> MASPPPFHSQKLPGEYFRYKGVPFPVGLYSLESISLAENTQDVRDDDIFIITYPKSGTTWMIEIICLILKEGDPSWIRSVPIWERAPWCETIVGAFSLPDQYSPRLMSSHLPIQIFTKAFFSSKAKVIYMGRNPRDVVVSLYHYSKIAGQLKDPGTPDQFLRDFLKGEVQFGSWFDHIKGWLRMKGKDNFLFITYEELQQDLQGSVERICGFLGRPLGKEALGSVVAHSTFSAMKANTMSNYTLLPPSLLDHRRGAFLRKGVCGDWKNHFTVAQSEA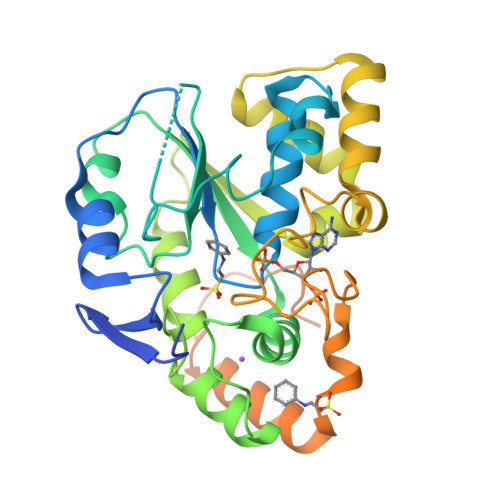FDRAYRKQMRGMPTFPWDEDPEEDGSPDPEPSPEPEPKPSLEPNTSLEREPRPNSSPSPSPGQASETPHPRPS ClfB, an MSCRAMM (Microbial Surface Components Recognizing Adhesive Matrix Molecules) family surface protein, described as a fibrinogen-binding clumping factor, is a key determinant of S. aureus nasal colonization, but the molecular basis for ClfB-ligand recognition remains unknown. ClfB plays a key role in establishing human nasal colonization by binding to the human type I cytokeratin 10 (CK10) expressed on squamous epithelial cells. As a bifunctional MSCRAMM, ClfB also binds to fibrinogen α (Fg α), which is assumed to be significant in platelet activation and aggregation and has been shown to contribute to the pathogenesis of experimental endocarditis in rats. In this study, we solved the crystal structures of apo-ClfB and its complexes with fibrinogen α (Fg α) and cytokeratin 10 (CK10) peptides.

To study the molecular mechanisms underlying ClfB-ligand recognition, we solved the crystal structures of ClfB(208–542) in complex with CK10 (amino acids 499–512, referred as CK10(499–512)) or Fg α (amino acids 316–328, referred as Fg α(316–328)) at 2.3 Å and 1.92 Å, respectively. In both complexes, the peptides adopt an extended conformation and are inserted into the tunnel formed between N2 and N3. Unlike Fg α(316–328), CK10(499–512) adopts a more extended conformation. In contrast with Fg α(316–328), the peptide CK10(499–512) did not induce formation of the β-strand G′ in ClfB. Nonetheless, the C-terminal portion of strand G that interacts with Fg α(316–328) also becomes well defined and caps on the CK10(499–512) peptide. Interestingly, although in the ClfB-CK10 structure the G′ strand appears disordered, the ClfBAsn238-Arg522 hydrogen bond also exists, consistent with the DLL model. In the ClfB(208–531)-CK10(499–512) complex structure, four pairs of hydrogen bonds were observed between the main chains of the peptide and the G strand of N3 domain, resulting in the formation of a parallel β-sheet. Polar groups in side chains of ClfBTrp522, and Asn524 in N3 domain form two hydrogen bonds with the hydroxyl group of CK10Ser503. The aromatic ring of ClfBTrp522 of the G strand of N3 plays an important role in anchoring the N-terminus of CK10 peptide through hydrophobic interactions with CK10Gly501 and CK10Gly502. Structural analysis showed that the space surrounding CK10Gly507 is significantly circumscribed by its neighboring residues ClfBVal528, Gly269, Val271, and Phe328.

> MRGSHHHHHHENLYFQGSLAVAEPVVNAADAKGTNVNDKVTASDFKLEKTAFDPNQSGNTFMAANFKVTGQVKSGDYFTAKLPDSVTGNGDVDYSNSNNTMPIADIKSTNGDVVAKATYDILTKTYTFVFTDYVNDKENINGQFSLPLFTDRAKAPKSGTYDANINIADEMFDNKITYNYSSPIAGIDKPNGANISSQIIGVDTASGQNTYKQTVFVNPKQRVLGNTWVYIKGYQDKIEESSGKVSATDTKLRIFEVNDTSKLSDSYYADPNDSNLKEVTGEFKDKISYKYDNVASINFGDINKTYVVLVEGHYDNTGKNLKTQVIQENIDPATGKDYSIFGWNNENVVRYGGGSADGDSAVN;> YGGGSSGGGSSGGG> MREYKVVVLGSGGVGKSALTVQFVTGTFIEKYDPTIEDFYRKEIEVDSSPSVLEILDTAGTEQFASM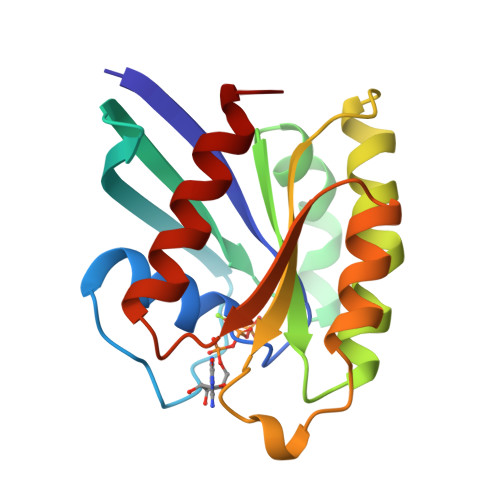RDLYIKNGQGFILVYSLVNQQSFQDIKPMRDQIIRVKRYEKVPVILVGNKVDLESEREVSSSEGRALAEEWGCPFMETSAKSKTMVDELFAEIVRQMNYA>[8x]MTAPTVPVALVTGAAKRLGRSIAEGLHAEGYAVCLHYHRSAAEANALSATLNARRPNSAITVQADLSNVATAPVSGADGSAPVTLFTRCAELVAACYTHWGR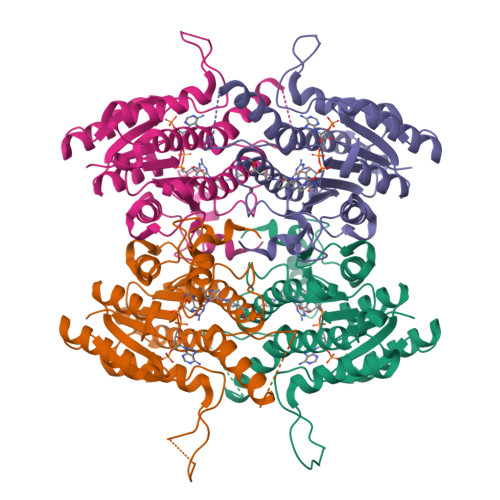CDVLVNNASSFYPTPLLRNDEDGHEPCVGDREAMETATADLFGSNAIAPYFLIKAFAHRVAGTPAKHRGTNYSIINMVDAMTNQPLLGYTIYTMAKGALEGLTRSAALELAPLQIRVNGVGPGLSVLVDDMPPAVWEGHRSKVPLYQRDSSAAEVSDVVIFLCSSKAKYITGTCVKVDGGYSLTRA methyl (2E)-{2-[(4-iodo-2,5-dimethylphenoxy)methyl]phenyl}(methoxyimino)ethanoate 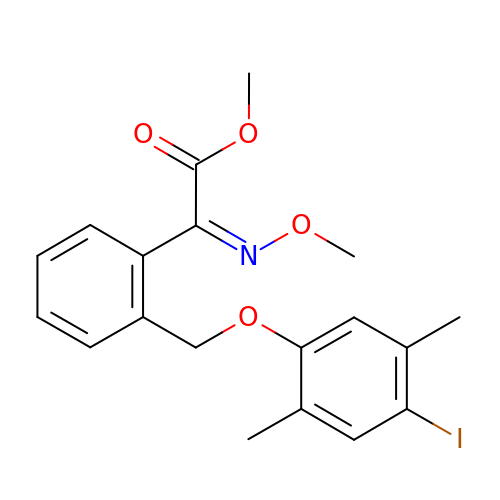| C19 H20 I N O4 | QNSHGJNFUSNVMK-DYTRJAOYSA-N> MVNRIELSRLIGLLLETEKRKNTEQKESGTNKIEDKVTLSK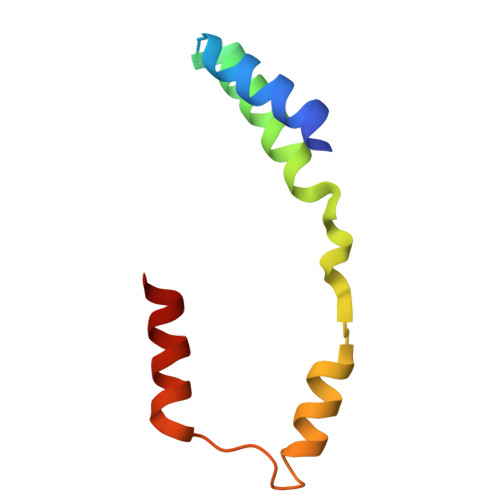IAQELSKNDVEEKDLEKKVKELKEKIEKGEYEVSDEKVVKGLIEFFT diethyl 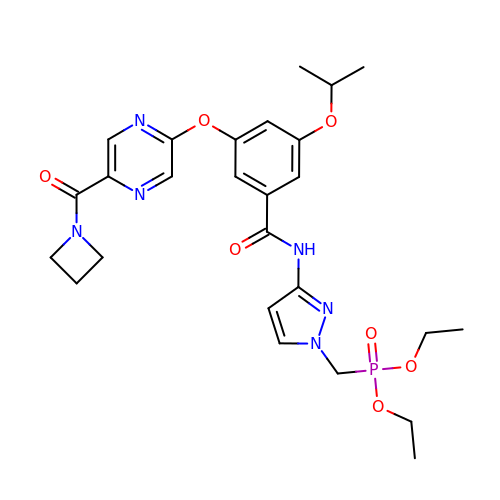{[3-(3-{[5-(azetidine-1-carbonyl)pyrazin-2-yl]oxy}-5-[(propan-2-yl)oxy]benzamido)-1H-pyrazol-1-yl]methyl}phosphonate | C26 H33 N6 O7 P | OYUDYQMFVRHPIY-UHFFFAOYSA-N> MGGHHHHHH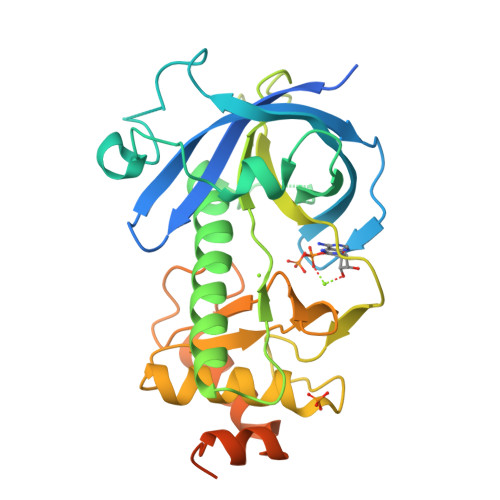GENLYFQGISSETGEMGILWEFDPIINKWIRLSMKLKVERKPFAEGALREAYHTVSLGVGTDENYPLGTTTKLFPPIEMISPISKNNEAMTQLKNGTKFVLKLYKKEAEQQASRELYFEDVKMQMVCRDWGNKFNQKKPPKKIEFLMSWVVELIDRSPSSNGQPILCSIEPLLVGEFKKNNSNYGAVLTNRSTPQAFSHFTYELSNKQMIVVDIQGVDDLYTDPQIHTPDGKGFGLGNLGKAGINKFITTHKCNAVCALLDLDVKLGGVLSGNNKKQLQQGTMVMPDILPELMPSDNT> PPHPQDLEITKLPNGLVIASLENYSPGSTIGVFIKAGSRYENSSNLGTSHLLRLASSLTTKGASSFKITRGIEAVGGKLSVESTRENMAYTVECLRDDVEILMEFLLNVTTAPEFRPWEVADLQPQLKIDKAVAFQNPQTHVIENLHAAAYRNALADSLYCPDYRIGKVTSVELHDFVQNHFTSARMALVGLG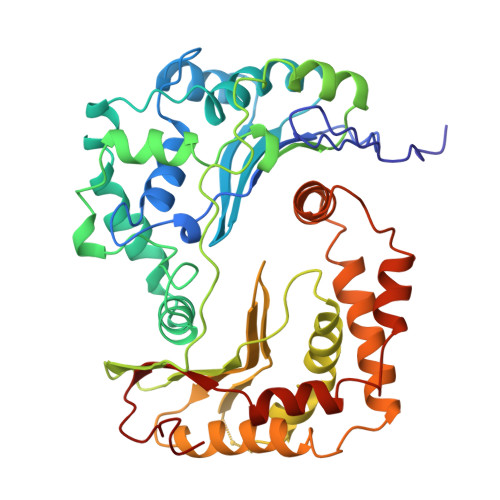VSHPVLKNVAEQLLNIRGGLGLSGAKAKYRGGEIREQNGDSLVHAAIVAESAAIGGAEANAFSVLQHVLGANPHVKRGLNATSSLYQAVAKGVHQPFDVSAFNASYSDSGLFGFYTISQAAYAGQVIKAAYNQVKTIAQGNVSNENVQAAKNKLKAKYLMSVESSEGFLEEVGSQALAAGSYNPPSTVLQQIDAVADADVIKAAKKFVSRQKSMAASGNLGHTPFVDEL>[2x]GSMSGNGNAAATAEENSPKMRVIRVGTRKSQLARIQTDSVVATLKASYPGLQFEIIAMSTTGDKILDTALSKIGEKSLFTKELEHALEKNEVDLVVHSLKDLPTVLPPGFTIGAICKRENPHDAVVFHPKFVGKTLETLPEKSVVGTSSLRRAAQLQRKFPHLEFRSIRGNLNTWLRKLDEQQEFSAIILATAGLQRMGWHNRVGQILHPEECMYAVGQGALGVEVRAKDQDILDLVGVLHDPETLLRCIAERAFLRHLEGGCSVPVAVHTAMKDGQLYLTGGVWSLDGSDSIQETMQATIHVPAQHEDGPEDDPQLVGITARNIPRGPQLAAQNLGISLANLLLSKGAKNILDVARQLNDAH

Porphobilinogen deaminase (PBGD; EC 2.5.1.61), also known as hydroxymethylbilane synthase (HMBS), is the third enzyme in the heme biosynthetic pathway. PBGD catalyzes four consecutive reactions to convert porphobilinogen (PBG) into hydroxymethylbilane (HMB), a linear tetrapyrrole heme precursor. The holoenzyme (Eholo) carries a dipyrromethane (DPM) cofactor, which is covalently linked to a conserved cysteine residue (Cys261 in hPBGD) through a thioether bond (Song et al., 2009). Mutations in the HMBS gene are associated with a genetic metabolic disorder known as acute intermittent porphyria (AIP), giving reduced heme production and severe metabolic and neurological symptoms (Bonkovsky et al., 2019).

The structure of the mutant R173W-hPBGD agrees with the ESI FT-ICR MS analysis, representing only ES2 in its reduced form (denoted R173W-ES2) and thus revealing for the first time an AIP-associated mutant trapped in a reaction intermediate state. The incorporation of S1 and S2 in R173W-ES2 causes a major rearrangement in the cofactor-binding loop Leu257–Val263 including Cys261 to which the reaction intermediate is covalently bound. In contrast to wt-Eholo, the active-site loop Ser57–Lys74 in R173W-ES2 is reoriented toward the C-terminal helix, α33, allowing the accommodation of the additional pyrrole rings in the active site cleft between the domains 1 and 2. Because of this rearrangement, the new pyrrole rings S1 and S2 take the original places of the C1 and C2 rings of the DPM cofactor in the wt-Eholo structure. The created cavity is not filled by the relocated C1 and C2 rings, and in the structure, a glycerol molecule occupies the space between C1 and the protein core. In R173W-ES2 presented here, the active-site loop is oriented in a significantly different conformation, partially facing away from the surface with Lys74 establishing several interactions with C2 and S1. Trp173 has different side chain conformations in the two subunits and has two alternative conformations in subunit A. We also discovered rearrangement in the helix α22 (residues 170–179) in subunit B. This rearrangement allows Trp173 to adopt a completely different conformation than seen in subunit A. From this point forward, we will only discuss the structure of subunit A, unless otherwise stated. The conformational change seen in subunit B of the R173W-ES2 structure, where the bulky tryptophan residue turns away from the active site forcing a change in the domain structure, probably also affects the loss in thermal stability. The substitution of Arg173 with tryptophan introduces a large hydrophobic amino acid, predicted to hinder the cofactor and/or substrate interaction severely. Both ESI FT-ICR MS and X-ray crystallography show that this mutant accumulates the ES2 intermediate with a greatly reduced turnover.> APATEETVIVEGSATAPDDGENDYSVTSTSAGTKMQMTQRDIPQSVTIVSQQRMEDQQLQTLGEVMENTLGISKSQADSDRALYYSRGFQIDNYMVDGIPTYFESRWNLGDALSDMALFERVEVVRGATGLMTGTGNPSAAINMVRKHATSREFKGDV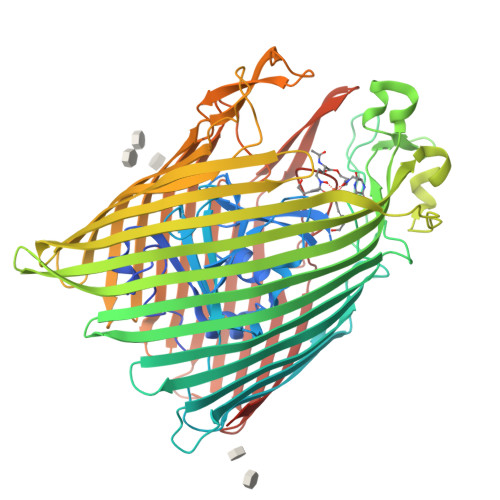SAEYGSWNKERYVADLQSPLTEDGKIRARIVGGYQNNDSWLDRYNSEKTFFSGIVDADLGDLTTLSAGYEYQRIDVNSPTWGGLPRWNTDGSSNSYDRARSTAPDWAYNDKEINKVFMTLKQQFADTWQATLNATHSEVEFDSKMMYVDAYVNKADGMLVGPYSNYGPGFDYVGGTGWNSGKRKVDALDLFADGSYELFGRQHNLMFGGSYSKQNNRYFSSWANIFPDEIGSFYNFNGNFPQTDWSPQSLAQDDTTHMKSLYAATRVTLADPLHLILGARYTNWRVDTLTYSMEKNHTTPYAGLVFDINDNWSTYASYTSIFQPQNDRDSSGKYLAPITGNNYELGLKSDWMNSRLTTTLAIFRIEQDNVAQSTGTPIPGSNGETAYKAVDGTVSKGVEFELNGAITDNWQLTFGATRYIAEDNEGNAVNPNLPRTTVKMFTSYRLPVMPELTVGGGVNWQNRVYTDTVTPYGTFRAEQGSYALVDLFTRYQVTKNFSLQGNVNNLFDKTYDTNVEGSIVYGTPRNFSITGTYQF>[8x]GSHMSYNNIPAGKDAPN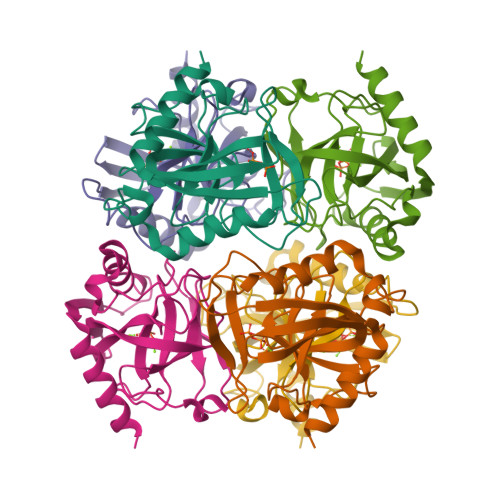DIYVIIEIPANAAPIKYEIDKDSDALFVDRFMGTAMFYPANYGYVPNTLSEDGDPLDVLVVTPYPVAAGSVIRCRPVGKLNMEDDGGIDAKLIAVPHEKLSPLYKDVKEYTDLPQLLINQVEHFFSHYKDLEPGKWVKISGWEGADVAKAEVIKAIEAAK>[2x]MIQGERLWQRLMELGEVGKQPSGGVTRLSFTAEERRAKDLVASYMREAGLFVYEDAAGNLIGRKEGTNPDATVVLVGSHLDSVYNGGCFDGPLGVLAGVEVVQTMNEHGVVTHHPIEVVAFTDEEGARFRFGM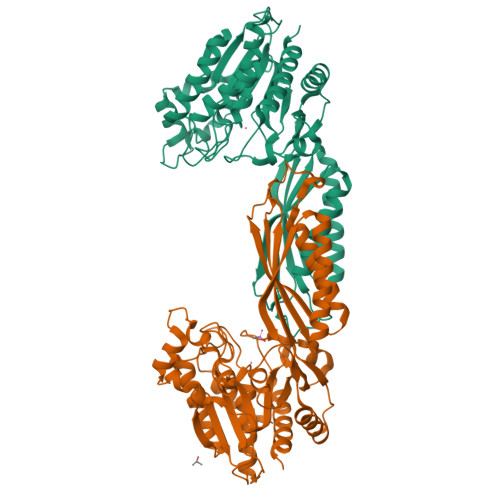IGSRAMAGTLPPEALECRDAEGISLAEAMKQAGLDPDRLPQAARKPGTVKAYVELHIEQGRVLEETGLPVGIVTGIAGLIWVKFTIEGKAEHAGATPMSLRRDPMAAAAQIIIVIEEEARRTGTTVGTVGQLHVYPGGINVIPERVEFVLDLRDLKAEVRDQVWKAIAVRAETIAKERNVRVTTERLQEMPPVLCSDEVKRAAEAACQKLGYPSFWLPSGAAHDSVQLAPICPIGMIFVRSQDGVSHSPAEWSTKEDCAAGAEVLYHTVWQLAQG> MKKYKIFTIAALLSSALVTTSCGDDFLTANSTEKPMAGAPATEGTILSSLGSAYQILLFDSYANNNYNSILLMSDLRSDDLYKGGGDAGDQAALYSLSQFNMSAAESLGGLWSIYFTGLARCNNAIIACANAEGVQERKVKQYNAEAHFLRAYYVHLLWKFFGNIPYFEEPLQDPYMTKQISADEIYNEIMADLEVACEEGVMEMVNNSGDNKGRACRAAALMLKARVVMYQKDQSRYAEIANDMATIIKSGKFELMDDFDAMWLDENEFCKESIFESNQLPEGKTWSSGWQ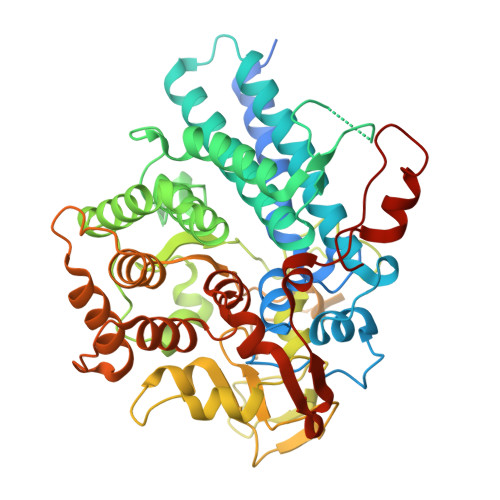GYGTNLPAFISPNELNDPSGVFKGGWGFAPVRQSAYDMYEEGDLRRDASINDWRGASYGHRFQDTGLFQRKYAAREGYNPPPGDTDLNYCNNLRIFRYAETLLNYVELVKMDGVAEQQGVDAQECFNLIRKRAFGIDKPLAATAENIKSERHKEFLGEGMRFYDLVRWGDAAAVLTENDAAHNSVRTYDDNKKLIPIPLNEIEKTKGTEFELKQNPGY> METMSEAQPQVISATGVVKGIDLESKK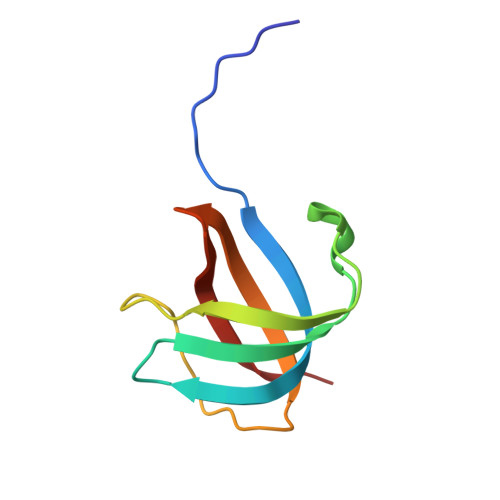ITIHHDPIAAVNWPEMTMRFTITPQTKMSEIKTGDKVAFNFVQQGNLSLLQDIKVSQ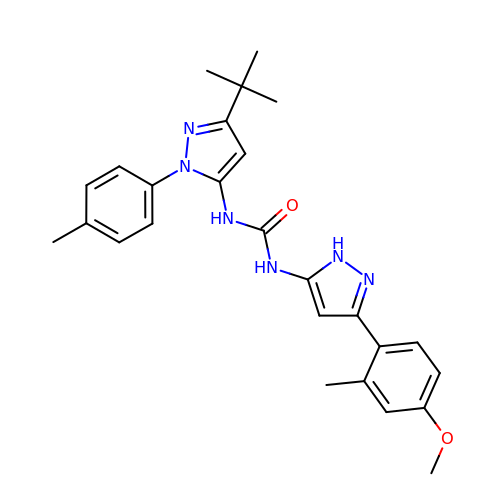1-[3-tert-butyl-1-(4-methylphenyl)-1H-pyrazol-5-yl]-3-[3-(4-methoxy-2-methylphenyl)-1H-pyrazol-5-yl]urea | C26 H30 N6 O2 | LATBWIWKSPOPNK-UHFFFAOYSA-N>MTSIEWDEKTFTKFAYLSDPRTRKNLVAYVLTKANLESNKYENTIVIENLEDGSRKFIEDASMPRISPDGKKIAFMRFNEEKKTAQIWVADLKTLSAKKVLEAKNIRSIEWNQDSRRLLAVGFKRREDEDFIFEDDVPAWFDNMGFFDGEKTTFWVIDTEGEEVIEQFEKPRFSSGIWHGDSIVVSVPHRDVIPRYFKYWDIYLWKDGEEEKLFEKVSFYAIDSDGERILLYGKPEKKYVSEHDKIYIYDGEVKGILDDIDREVAQAKIRNGKVYFTLFEEGSVNLYLWDGEVREIAKGKHWIMGFDADERLIYLKETATRPAELYLWDGEERQLTDYNGLIFKKLKTFEPRHFRFKSIDLELDGWYIKPEIKEGEKAPVIVFVHGGPKGMYGYYFKYEMQLMASKGYYIVYVNPRGSNGYSEDFALRVLERTGLEDFQDILNGIEEFLRLEPQADRERIGITGIAYGGYMTNWALTQSDLFKAGISENGISYWLTSYAFSDIGLWFDKEVIGDNPLENENYRKLSPLFYAKNVKAPLLLIHSLEDYRCPLDQSLMFYHVLKDLGKEVYIAIFKKGAHGHSIRGSPRHRMKRYKLFMEFFERKLKKYEEGFDVEKIL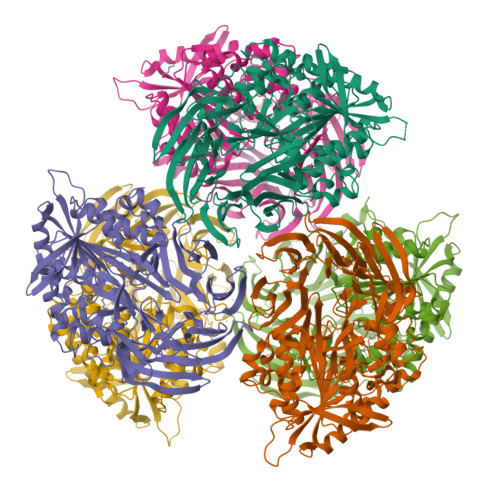KEEKK[12x]>[2x]A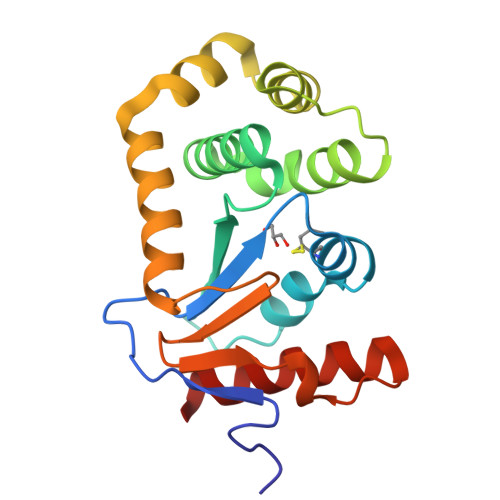QYEDGKQYTTLEKPVAGAPQVLEFFSFFCPHCYQFEEVLHISDNVKKKLPEGVKMTAYHVNFMGGDLGKDLTQAWAVAMALGVEDKVTVPLFEGVQKTQTIRSASDIRDVFINAGIKGEEYDAAWNSFVVKSLVAQQEKAAADVQLRGVPAMFVNGKYQLNPQGMDTSNMDVFVQQYADTVKYLSEKK>MGLSLPKEKGLILCLWSKFCRWFQRRESWAQSRDEQNLLQQKRIWESPLLLAAKDNDVQALNKLLKYEDCKVHQRGAMGETALHIAALYDNLEAAMVLMEAAPELVFEPMTSELYEGQTALHIAVVNQNMNLVRALLARRASVSARATGTAFRRSPCNLI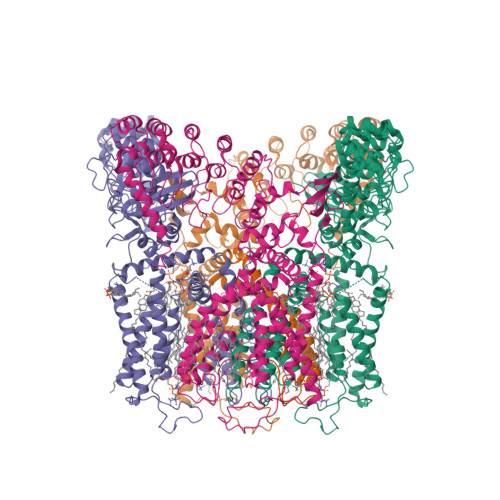YFGEHPLSFAACVNSEEIVRLLIEHGADIRAQDSLGNTVLHILILQPNKTFACQMYNLLLSYDRHGDHLQPLDLVPNHQGLTPFKLAGVEGNTVMFQHLMQKRKHTQWTYGPLTSTLYDLTEIDSSGDEQSLLELIITTKKREARQILDQTPVKELVSLKWKRYGRPYFCMLGAIYLLYIICFTMCCIYRPLKPRTNNRTSPRDNTLLQQKLLQEAYMTPKDDIRLVGELVTVIGAIIILLVEVPDIFRMGVTRFFGQTILGGPFHVLIITYAFMVLVTMVMRLISASGEVVPMSFALVLGWCNVMYFARGFQMLGPFTIMIQKMIFGDLMRFCWLMAVVILGFASAFYIIFQTEDPEELGHFYDYPMALFSTFELFLTIIDGPANYNVDLPFMYSITYAAFAIIATLLMLNLLIAMMGDTHWRVAHERDELWRAQIVATTVMLERKLPRCLWPRSGICGREYGLGDRWFLRVEDRQDLNRQRIQRYAQAFHTRGSEDLDKDSVEKLVPR[4x]>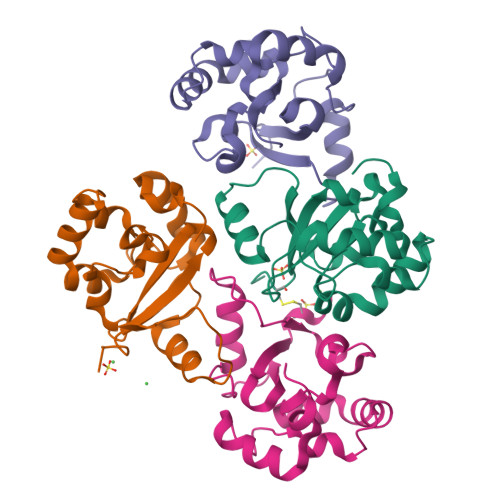[4x]SCGCHEAIMAILPECNGIMITTRDHAGMTPSGMTFSTLAGMIGGGTQTPGFMGIGRTYIVSKKFISADGGIARIVWMPKSLKDFLHDEFVRRSVEEGLGEDFIDKIADETIGTTVDEILPYLEEKGHPALTMDPI>[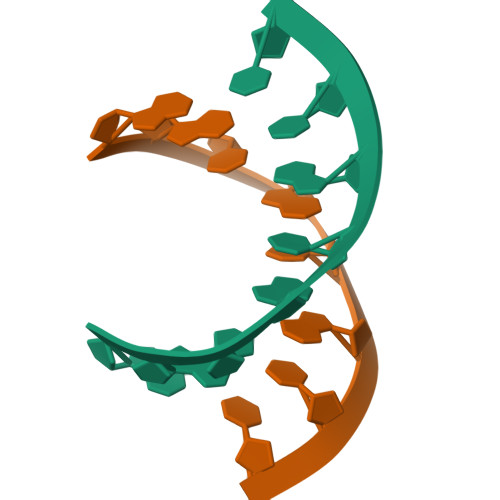10x]GGCGUGCC(3S)-3-(methylamino)-1-phenylpiperidin-2-one | C12 H16 N2 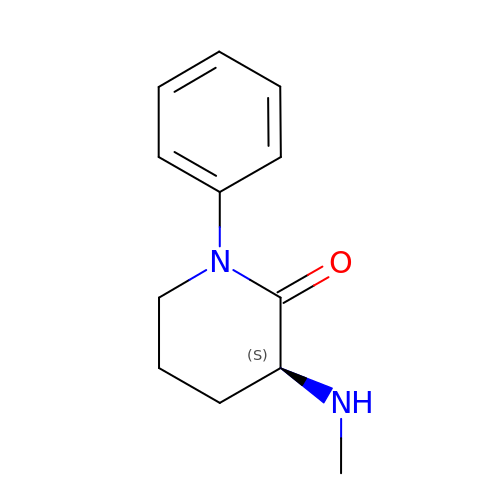O | PVGKKAFLCYRCCI-NSHDSACASA-N In this study, a series of 20S(OH)D3 analogs with modified side chains were chemically synthesized. The crystal structures of 20S(OH)D3, 4 and 33 analogs in complex with the Danio Rerio VDR (zVDR) LBD were determined and compared to those of 1,20S(OH)2D3 and 1,25(OH)2D3 VDR complexes. Co-crystal structures of VDR in complex with 20S(OH)D3, 4, and 33 revealed notable differences in their molecular interactions in the binding pocket of VDR, which will be insightful for developing novel VDR agonists as anti-inflammatory agents.

Two analogs (4 and 33) were chosen to co-crystalize with the VDR to decipher their differential modes of interaction in comparison with 20S(OH)D3 and 1,25(OH)2D3. The modifications included replacing C24 with an oxygen, inserting a double bond between C24 and C25 (4), adding an amide group replacing carbons 23 and 24 (33) and adding two fluorine groups at C24 (23). Similarly, the D3-like structure 33 having a 23-amide modification was obtained from the the photochemical opening of the B-ring. Analogs 4 and 33 cause conformational changes in the position of His305 and His397 with quite a substantial change in the case of 33 which formed a hydrogen bond between His397 and the amide group which is in contrast to 20S(OH)D3 which does not interact with this residue. While the exact relationship between these conformational changes induced by 33 and VDR function remain to be elucidated, the change indicates the possibility of producing analogs that display a unique subset of the actions seen for 1,25(OH)2D3 (i.e. are biased agonists), as already seen to some degree for the parental 20S(OH)D3. In contrast, the introduction of an amide linkage into the side chain, as in 33, prevented its hydroxylation by CYP27B1. All analogs tested except 33 were metabolized by CYP27B1. 20S(OH)D3 and 33 displayed similar catalytic efficiencies which were the lowest of the analogs tested and 13-fold lower than for 13.

> GSHMLSDEQMQIINSLVEAHHKTYDDSYSDFVRFRPPVREGPVTRSASRAASLHSLSDASSDSFNHSPESVDTKLNFSNLLMMYQDSGSPDSSEEDQQSRLSMLPHLADLVSYSIQKVIGFAKMIPGFRDLTAEDQIALLKSSAIEIIMLRSNQSFSLEDMSWSCGGPDFKYCINDVTKAGHTLELLEPLVKFQVGLKKLKLHEEEHVLLMAICLLSPDRPGVQDHVRIEALQDRLCDVLQAYIRIQHPGGRLLYAKMIQKLADLRSLNEEHSKQYRSLSFQPEHSMQLTPLVLEVFGSEVS;> RHKILHRLLQEGSPS> GGGRMEVAEANSPTEEEEEEEEEGEETISEPRPHTRSNPEGAEDRALGAQASVGSRSEGEGEAATADGGAASVPGAGPKPWQVPASASEVQIRTPRVNCPEKVIICLDLSEEMSVPKLESFNGSRTNALNVSQKMVEMFVRTKHKIDKSHEFALVVVNDDSAWLSGLTSDPRELCSCLYDLETASCSTFNLEGLFSLIQQKTELPVTENVQTIPPPYVVRTILVYSRPPCQPQFSLTEPMKKMFQCPYFFFDIVYIHNGTEEKEE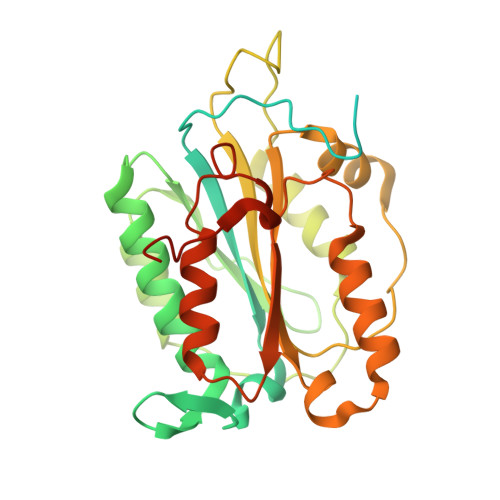DMSWKDMFAFMGSLDTKGASYKYEVALAGPALELHNCMAKLLAHPLQRPCQTHASYSLLEEDEEAGEEEATV> MGSDKIHHHHHHMVYVGTSGFSFEDWKGVVYPEHLKPSQFLKYYWAVLGFRIVELNFTYYTQPSWRSFVQMLRKTPPDFYFTVKTPGSVTHVL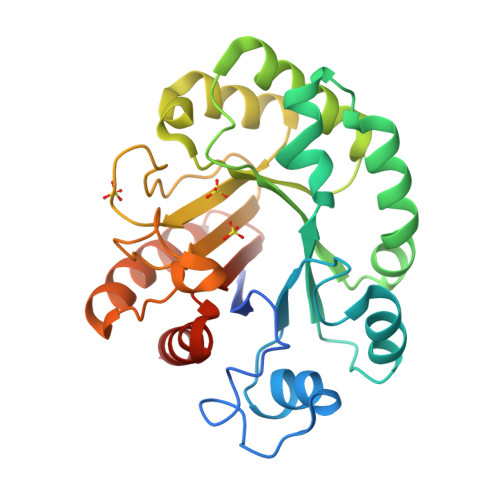WKEGKDPKEDMENFTRQIEPLIEEQRLKMTLAQFPFSFKFSRKNVEYLEKLRESYPYELAVEFRHYSWDREETYEFLRNHGITFVVVDEPKLPGLFPYRPITTTDYAYFRFHGRNERWFEAEGEERYDYLYSEEELKTLFEDVVELSRRVKETYVFFNNCYKGQAAINALQFKKMLEERV>ASNFTQFVLVDNGGTGDVTVAPSNFANGVAEWISSNSRSQAYKVACSVRQSSAQNRKYTIKVEVPKVATQTVGGVELPVAAWRSYLNMELTIPIFATNSDCELIVKAMQGLLKDGNPIPSAIAANSG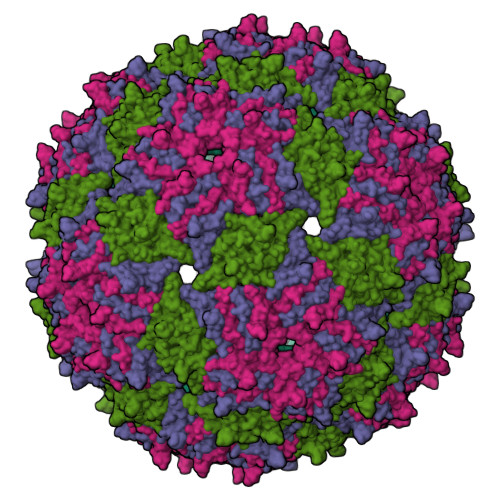IY[3x]> GPGGSGGVTEEQVHHIVKQALQRYSEDRIGLADYALESGGASVISTRCSETYETKTALLSLFGIPLWYHSQSPRVILQPDVHPGNCWAFQGPQGFAVVRLSARIRPTAVTLEHVPKALSPNSTISSAPKDFAIFGFDEDLQQEGTLLGKFTYDQDGEPIQ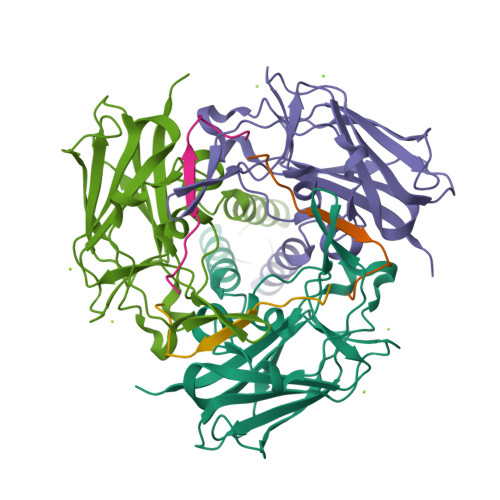TFHFQAPTMATYQVVELRILTNWGHPEYTCIYRFRVHGEPAH;> GPGGSGSGGPCCSHARIPRTPYLVLSYVNGLPPV>[8x]MTDVVIVSAARTAVGKFGGSLAKIPAPELGAVVIKAALERAGVKPEQVSEVIMGQVLTAGSGQNPARQAAIKAGLPAMVPAMTINKVSGSGLKAVMLAANAIMAGDAEIVVAGGQENMSAAPHVLPGSRDGFRMGDAKLVDTMIVDGLWDVYNQYHMGITAENVAKEYGITREAQDEFAVGSQNKAEAAQKAGKFDEEIVPVLIPQRKGDPVAFK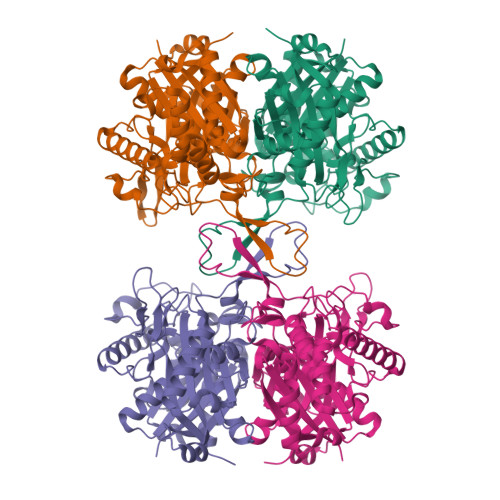TDEFVRQGATLDSMSGLKPAFDKAGTVTAANASGLNDGAAAVVVMSAAKAKELGLTPLATIKSYANAGVDPKVMGMGPVPASKRALSRAEWTPQDLDLMEINEAFAAQALAVHQQMGWDTSKVNVNGGAIAIGHPIGASGCRILVTLLHEMKRRDAKKGLASLCIGGGMGVALAVERK> MKQLLIVDDQQGIRLLLNEVFKREGYTTFLAANGIEALDIAERVKPDGVLL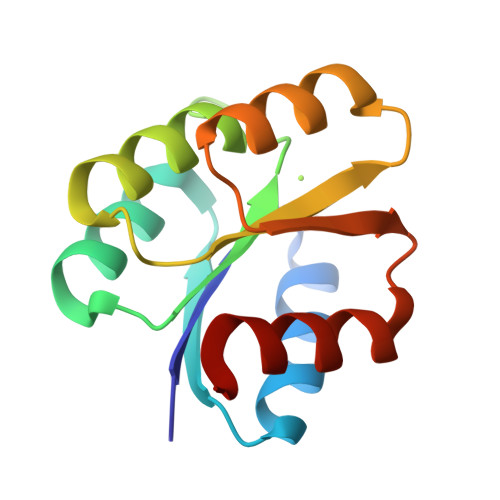DMKIPGMDGIEILKRIKTRTPDVPVLMMTAYGELDLIKEAMDLGASHYFTKPFDIYELRDAVNEMLRD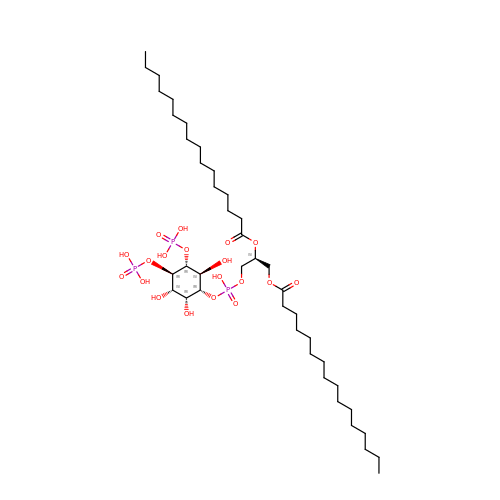(2S)-3-{[(R)-hydroxy{[(1R,2R,3S,4R,5R,6S)-2,3,6-trihydroxy-4,5-bis(phosphonooxy)cyclohexyl]oxy}phosphoryl]oxy}propane-1,2-diyl dihexadecanoate | C41 H81 O19 P3 | HKWJHKSHEWVOSS-MVLQGUJPSA-N>MIDQSDWISFSHMSSDTDHFPIKSWFRCEQKAASRSYRTLGDMSHPQGIYEVRAAITRLISLTRGVKCRPEQMIIGAGTQVLMQLLTELLPKEAVYAMEEPGYRRMYQLLKNAGKQVKTIMLDEKGMSIAEITRQQPDVLVTTPSHQFPSGTIMPVSRRIQLLNWAAEEPRRYIIEDDYDSEFTYDVDSIPALQSLDRFQNVIYMGTFSKSLLPGLRISYMVLPPELLRAYKQRGYDLQTCSSLTQLTLQEFIE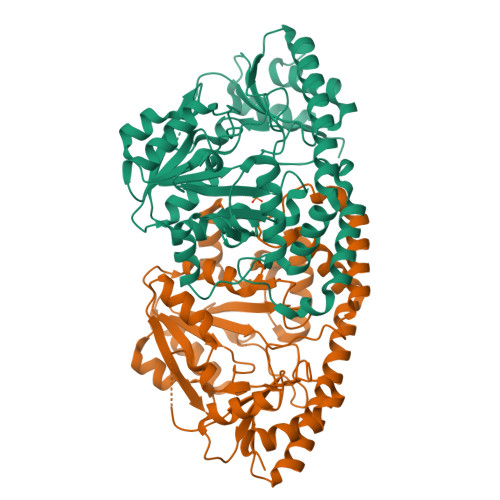SGEYQKHIKKMKQHYKEKRERLITALEAEFSGEVTVKGANAGLHFVTEFDTRRTEQDILSHAAGLQLEIFGMSRFNLKENKRQTGRPALIIGFARLKEEDIQEGVQRLFKAVYGHKKIPVTGDHHHHHH[2x]>SNAMLKDIHQHRILILDFGSQYAQLIARRVREIGVYCELMPCDIDEETIRDFNPHGIILSGGPETVTLSHTLRAPAFIFEIGCPVLGICYGMQTMAYQLGGKVNRTAKAEFGHAQLRVLNPAFLFDGIEDQVSPQGEPLLDVWMSHGDIVSELPPGFEATACTDNSPLAAMADFKRRFFGLQFHPEVTHTPQGHRILAHFVIHICQCIPNWTTKHIIEDSIRDIQEKVGKEQVIVGLSGGVDSAVTATLVHKAIGDQLVCVLVDTGLLRLNEVDEVLNVFQKHLGAKVICVDAKDRFM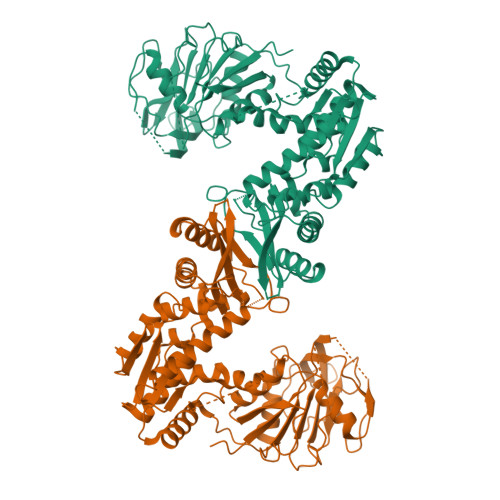KALKGISDPEEKRKIAGEQFIRVFEEQAKKLNVKWLGQGTIYPDVIESAKTKTGKGHIIKTHHNVGGLPLNMELKLIEPLRELFKDEVRKLGLELGLPADLIYRHPFPGPGLAIRILGEVSAEYINILKQADAIFIEELKKSDYYHQVSQAFAVFMPLKSVGVKGDARHYGYIIALRAVKTVDFMTAQWADLPHEFLSKVSHRIVNEIKEVSRVVYDMTNKPPATIEWE[4x]7-ALPHA-D-RIBOFURANOSYL-2-AMINOPURINE-5'-PHOSPHATE | C10 H14 N5 O7 P | 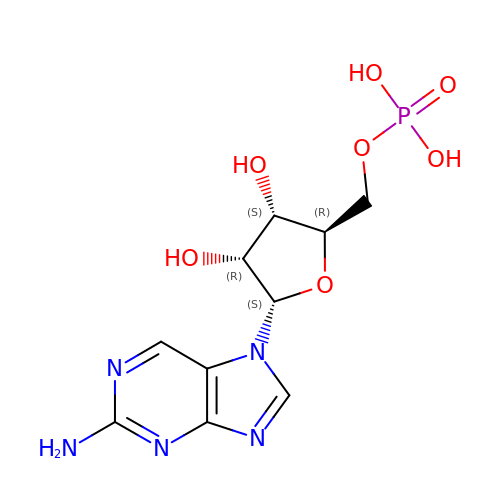UDRQVOJQMHZSIM-PULFBKJNSA-N3,5-bis(fluoranyl)-~{N}-[3-[(2-fluoranyl-4-methoxy-phenyl)sulfamoyl]phenyl]benzamide 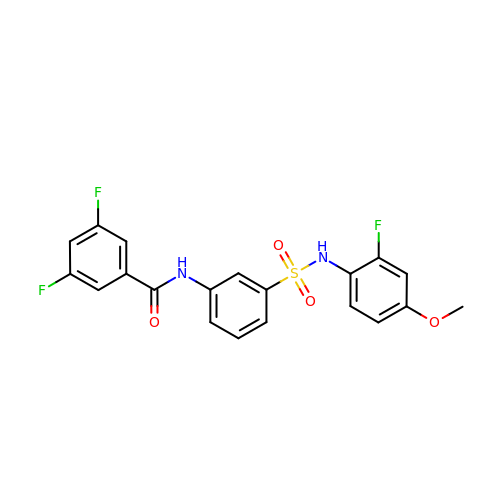| C20 H15 F3 N2 O4 S | NWMPDNCLCRMZII-UHFFFAOYSA-N>EAEAEFQTSCEQYAVFSGGNGYSVSNNLWGQSAGSGFGCITVNSLNSAASWHADWQWSGGQNNVKSYPNVQIAIPQKRIVNSIGSMPTTASWSYTGSNLRADVAYDLFTASNPNHVTYSGDYELMIWLARYGDIGPIGSAQGTVTINGQSWTLYYGFNGAMQVYSFVAPSTVTNWSGDVKNFFNYLRDNKGYPASSQYVLSYQFGTEPFTGSGTLNVNSWTASINV[2x]

The endoglucanase 3 (known also as Cel12A) of Trichoderma reesei (TrEG3) and Trichoderma harzianum (ThEG3) constitute an example of these CBM-less enzymes. On the other hand, these enzymes are particularly active in the amorphous regions of cellulose or in the hydrolysis of soluble oligosaccharides, which suggests that the catalytic core of these enzymes not only possesses the catalytic functions, but might also bear CBM-like motifs specific for interactions with amorphous regions of the substrate. In this study, we report the three-dimensional structure of ThEG3 obtained from X-ray crystallography and investigate enzyme-substrate interactions using molecular dynamics (MD) simulations. We identify amino acids at the body of Cel12A that play key roles in substrate binding and, thus, provide a structural basis for the fact that Cel12A enzymes relinquish a cellulose-binding module.

We solved the crystallographic structure of endoglucanase 3 from Trichoderma harzianum at 2.07 Å resolution and performed molecular dynamics simulations on this new structure with the aim to shed more light on the Cel12A dynamics and its binding mechanism oligosaccharides. The β-strands are connected via several loops and three α-helices (H1, H2 and H3). The concave part of the leaflets constitutes the catalytic cleft, which binds to the cellulose chains during the hydrolysis. Figure 1D shows the catalytic residues Asp100, Glu117, and Glu201, strictly conserved in the glycosyl hydrolase family 12. The distance of 5.6 Å between Glu117 and Glu201 is typical for the nucleophile/acid catalyst pairs involved in the hydrolysis mechanism that gives rise to retention of the anomeric configuration of the reaction product. The ThEG3 is composed by 220 residues and has high primary sequence identity (83%) with TrEG3, with just two additional residues. Like TrEG3, there is an evident row of hydrophobic residues in one of the edges of the cleft, formed by Tyr7, Trp23, Val58, Phe203, and Ile128. Close to the acid catalyst Glu201, ThEG3 has another acid residue, Asp96, whereas TrEG3 has Asn95. The simulations suggest that a CBM-like cluster of key residues located in the loops at one end of the catalytic cleft is responsible for recognizing and binding the polymeric substrate.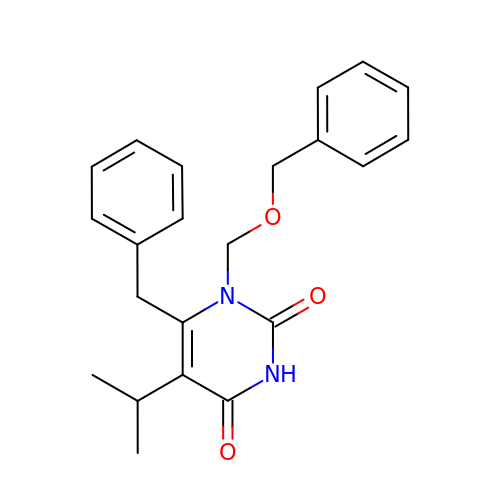6-BENZYL-1-BENZYLOXYMETHYL-5-ISOPROPYL URACIL | C22 H24 N2 O3 | KSAAUHMSLCPIEX-UHFFFAOYSA-N> DRPRFSFSIAAREGKARTGTIEMKRGVIRTPAFMPVGTAATVKALKPETVRATGADIILGNTYHLMLRPGAERIAKLGGLHSFMGWDRPILTDSGGYQVMSLSSLTKQSEEGVTFKSHLDGSRHMLSPERSIEIQHLLGSDIVMAFDECTPYPAT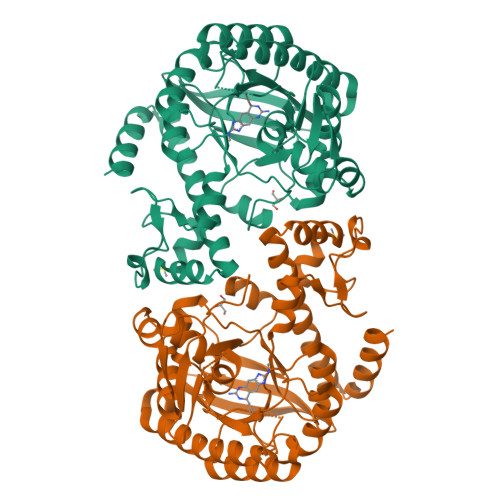PSRAASSMERSMRWAKRSRDAFDSRKEQAENAALFGIQQGSVFENLRQQSADALAEIGFDGYAVGGLAVGEGQDEMFRVLDFSVPMLPDDKPHYLMGVGKPDDIVGAVERGIDMFDCVLPTRSGRNGQAFTWDGPINIRNARFSEDLKPLDSECHCAVCQKWSRAYIHHLIRAGEILGAMLMTEHNIAFYQQLMQKIRDSISEGRFSQFAQDFRARYFAR>[6x]MNDYSRQNFLDLNLFR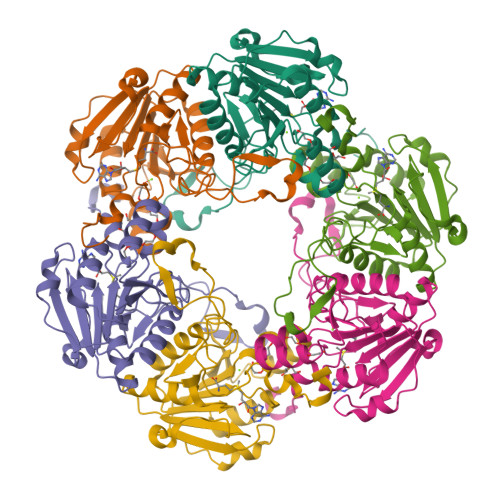GLGEDPAYHPPVLTDRPRDWPLDRWAEAPRDLGYSDFSPYQWRGLRMLKDPDTQAVYHDMLWELRPRTIVELGVYNGGSLAWFRDLTKIMGIDCQVIGIDRDLSRCQIPASDMENITLHQGDCSDLTTFEHLREMAHPLIFIDDAHANTFNIMKWAVDHLLEEGDYFIIEDMIPYWYRYAPQLFSEYLGAFRDVLSMDMLYANASSQLDRGVLRRVAAKQ>DNYIYSTEVGGVGGTPFTFMQESGTITSIKFNWSDQYKLLHHIEVKFIN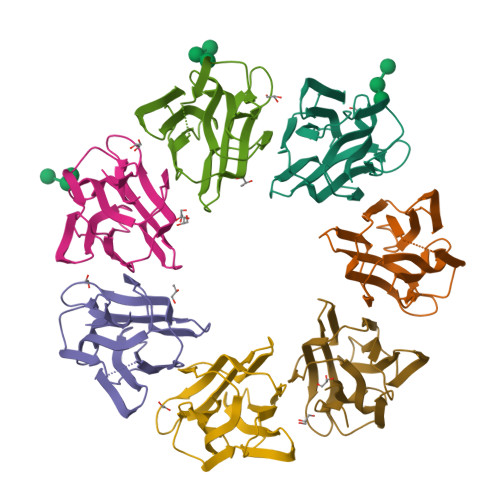NANIYATGDPKGNHEVILEIDDDETIIGSVIGYKKGNDGRCTGVKLTTSKGKSIMAGYFEESLITTYTGKLAGIKGGAGSDIDRLGLIFLK[7x]>[4x]MTDTYLHETLVFDNKLSYIDNQRDT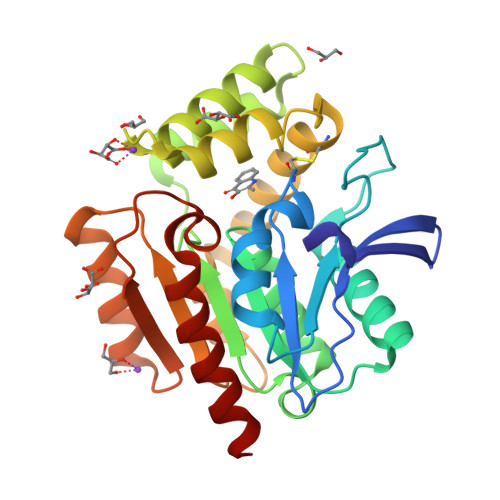DGPAILLLPGWCHDHRVYKYLIQELDADFRVIVPNWRGHGLSPSEVPDFGYQEQVKDALEILDQLGVETFLPVSHSHGGWVLVELLEQAGPERAPRGIIMDWLMWAPKPDFAKSLTLLKDPERWREGTHGLFDVWLDGHDEKRVRHHLLEEMADYGYDCWGRSGRVIEDAYGRNGSPMQMMANLTKTRPIRHIFSQPTEPEYEKINSDFAEQHPWFSYAKLGGPTHFPAIDVPDRAAVHIREFATAIRQGQ> GKITLYEDRGFQGRHYECSSDHPNLQPYLSRCNSARVDSGCWMLYEQPNYSGLQYFLRRGDYADHQQWMGLSDSVRSCRLIPHSGSHRIRLYEREDYRGQMIEFTEDCSCLQDRFRFNEIHSLDVLEGSWVLYELSNYRG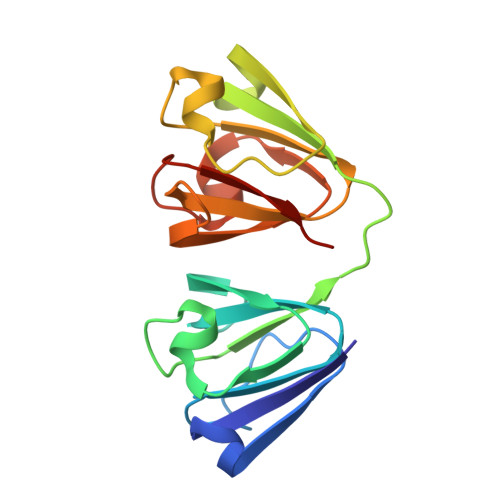RQYLLMPGDYRRYQDWGATNARVGSLRRVIDFS>MEGMLKGEGPGPLPPLLQQYVELRDQYPDYLLLFQVGDFYECFGEDAERLARALGLVLTHKTSKDFTTPMAGIPLRAFEAYAERLLKMGFRLAVADQVEPAEEAEGLVRREVTQLLTPGTLLQESLLPREANYLAAIATGDGWGLAFLDVSTGEFKGTVLKSKSALYDEL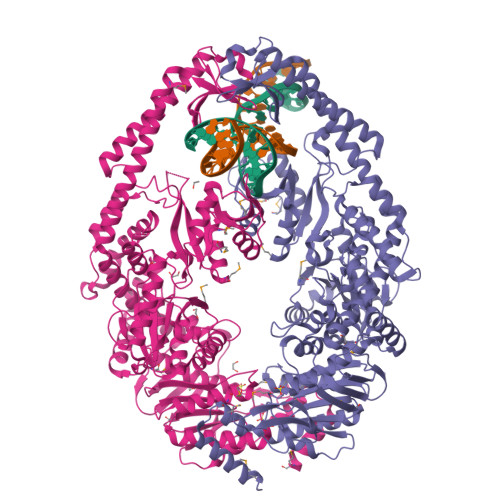FRHRPAEVLLAPELLENGAFLDEFRKRFPVMLSEAPFEPEGEGPLALRRARGALLAYAQRTQGGALSLQPFRFYDPGAFMRLPEATLRALEVFEPLRGQDTLFSVLDETRTAPGRRLLQSWLRHPLLDRGPLEARLDRVEGFVREGALREGVRRLLYRLADLERLATRLELGRASPKDLGALRRSLQILPELRALLGEEVGLPDLSPLKEELEAALVEDPPLKVSEGGLIREGYDPDLDALRAAHREGVAYFLELEERERERTGIPTLKVGYNAVFGYYLEVTRPYYERVPKEYRPVQTLKDRQRYTLPEMKEKEREVYRLEALIRRREEEVFLEVRERAKRQAEALREAARILAELDVYAALAEVAVRYGYVRPRFGDRLQIRAGRHPVVERRTEFVPNDLEMAHELVLITGPNMAGKSTFLRQTALIALLAQVGSFVPAEEAHLPLFDGIYTRIGASDDLAGGKSTFMVEMEEVALILKEATENSLVLLDEVGRGTSSLDGVAIATAVAEALHERRAYTLFATHYFELTALGLPRLKNLHVAAREEAGGLVFYHQVLPGPASKSYGVEVAAMAGLPKEVVARARALLQAMAAR[2x]>LVYFAAXLK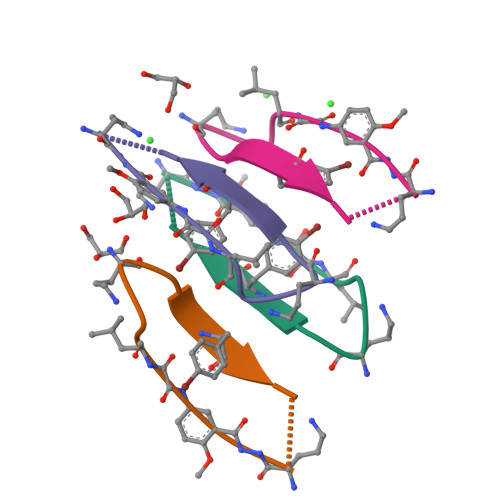A[8x]> MDEEEDGAGAEESGQPRSFMRLNDLSGAGGRPGPGSAEKDPGSADSEAEGLPYPALAPVVFFYLSQDSRPRSWCLRTVCNPWFERISMLVILLNCVTLGMFRPCEDIACDSQRCRILQAFDDFIFAFFAVEMVVKMVALGIFGKKCYLGDTWNRLDFFIVIAGMLEYSLDLQNVSFSAVRTVRVLRPLRAINRVPSMRILVTLLLDTLPMLGNVLLLCFFVFFIFGIVGVQLWAGLLRNRCFLPENFSLPLSVDLERYYQTENEDESPFICSQPRENGMRSCRSVPTLRGDGGGGPPCGLDYEAYNSSSNTTCVNWNQYYTNCSAGEHNPFKGAINFDNIGYAWIAIFQVITLEGWVDIMYFVMDAHSFYNFIYFILLIIVGSFFMINLCLVVIATQFSETKQRESQLMREQRVRFLSNASTLASFSEPGSCYEELLKYLVYILRKAARRLAQVSRAAGVRVGLLSSPAPLGGQETQPSSSCSRSHRRLSVHHLVHHHHHHHHHYHLGNGTLRAPRASPEIQDRDANGSRRLMLPPPSTPALSGAPPGGAESVHSFYHADCHLEPVRCQAPPPRSPSEASGRTVGSGKVYPTVHTSPPPETLKEKALVEVAASSGPPTLTSLNIPPGPYSSMHKLLETQSTGACQSSCKISSPCLKADSGACGPDSCPYCARAGAGEVELADREMPDSDSEAVYEFTQDAQHSDLRDPHSRRQRSLGPDAEPSSVLAFWRLICDTFRKIVDSKYFGRGIMIAILVNTLSMGIEYHEQPEELTNALEISNIVFTSLFALEMLLKLLVYGPFGYIKNPYNIFDGVIVVISVWEIVGQQGGGLSVLRTFRLMRVLKLVRFLPALQRQLVVLMKTMDNVATFCMLLMLFIFIFSILGMHLFGCKFASERDGDTLPDRKNFDSLLWAIVTVFQILTQEDWNKVLYNGMASTSSWAALYFIALMTFGNYVLFNLLVAILVEGFQAEGDANKSESEPDFFSPSLDGDGDRKKCLALVSLGEHPELRKSLLPPLIIHTAATPMSLPKSTSTGLGEALGPASRRTSSSGSAEPGAAHEMKSPPSARSSPHSPWSAASSWTSRRSSRNSLGRAPSLKRRSPSGERRSLLSGEGQESQDEEESSEEERASPAGSDHRHRGSLEREAKSSFDLPDTLQVPGLHRTASGRGSASEHQDCNGKSASGRLARALRPDDPPLDGDDADDEGNLSKGERVRAWIRARLPACCLERDSWSAYIFPPQSRFRLLCHRIITHKMFDHVVLVIIFLNCITIAMERPKIDPHSAERIFLTLSNYIFTAVFLAEMTVKVVALGWCFGEQAYLRSSWNVLDGLLVLISVIDILVSMVSDSGTKILGMLRVLRLLRTLRPLRVISRAQGLKLVVETLMSSLKPIGNIVVICCAFFIIFGILGVQLFKGKFFVCQGEDTRNITNKSDCAEASYRWVRHKYNFDNLGQALMSLFVLASKDGWVDIMYDGLDAVGVDQQPIMNHNPWMLLYFISFLLIVAFFVLNMFVGVVVENFHKCRQHQEEEEARRREEKRLRRLEKKRRNLMLDDVIASGSSASAASEAQCKPYYSDYSRFRLLVHHLCTSHYLDLFITGVIGLNVVTMAMEHYQQPQILDEALKICNYIFTVIFVLESVFKLVAFGFRRFFQDRWNQLDLAIVLLSIMGITLEEIEVNASLPINPTIIRIMRVLRIARVLKLLKMAVGMRALLDTVMQALPQVGNLGLLFMLLFFIFAALGVELFGDLECDETHPCEGLGRHATFRNFGMAFLTLFRVSTGDNWNGIMKDTLRDCDQESTCYNTVISPIYFVSFVLTAQFVLVNVVIAVLMKHLEESNKEAKEEAELEAELELEMKTLSPQPHSPLGSPFLWPGVEGPDSPDSPKPGALHPAAHARSASHFSLEHPTMQPHPTELPGPDLLTVRKSGVSRTHSLPNDSYMCRHGSTAEGPLGHRGWGLPKAQSGSVLSVHSQPADTSYILQLPKDAPHLLQPHSAPTWGTIPKLPPPGRSPLAQRPLRRQAAIRTDSLDVQGLGSREDLLAEVSGPSPPLARAYSFWGQSSTQAQQHSRSHSKISKHMTPPAPCPGPEPNWGKGPPETRSSLELDTELSWISGDLLPPGGQEEPPSPRDLKKCYSVEAQSCQRRPTSWLDEQRRHSIAVSCLDSGSQPHLGTDPSNLGGQPLGGPGSRPKKKLSPPSITIDPPESQGPRTPPSPGI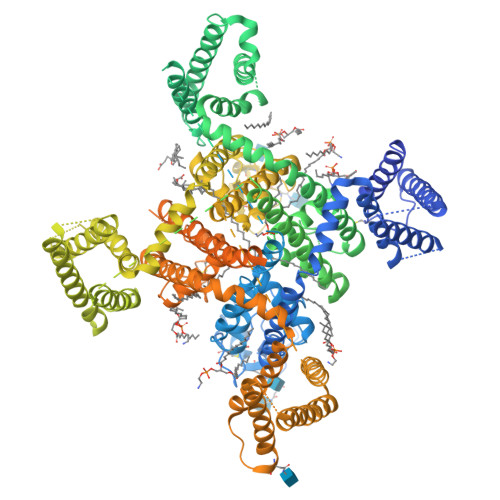CLRRRAPSSDSKDPLASGPPDSMAASPSPKKDVLSLSGLSSDPADLDP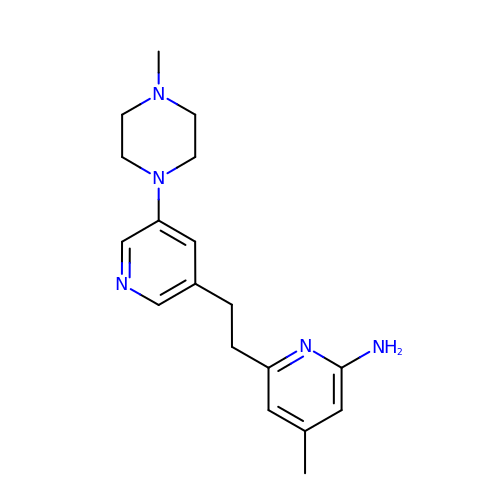4-methyl-6-(2-(5-(4-methylpiperazin-1-yl)pyridin-3-yl)ethyl)pyridin-2-amine | C18 H25 N5 | QJETXLUKROHQMG-UHFFFAOYSA-N>[6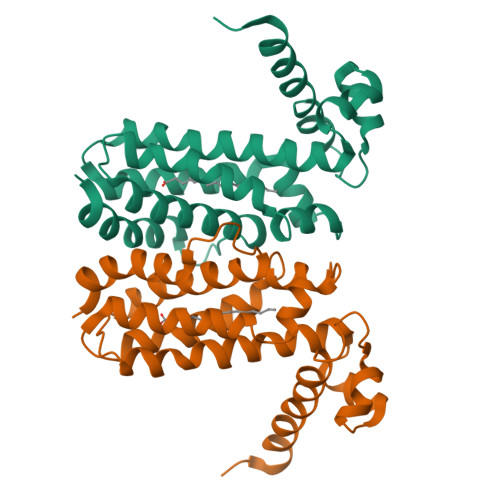x]MSTPSATVAPVKRIPYAEASRALLRDSVLDAMRDLLLTRDWSAITLSDVARAAGISRQTIYNEFGSRQGLAQGYALRLADRLVDNVHASLDANVGNFYEAFLQGFRSFFAESAADPLVISLLTGVAKPDLLQLITTDSAPIITRASARLAPAFTDTWVATTDNDANVLSRAIVRLCLSYVSMPPEADHDVAADLARLITPFAERHGVINVPHHHHHH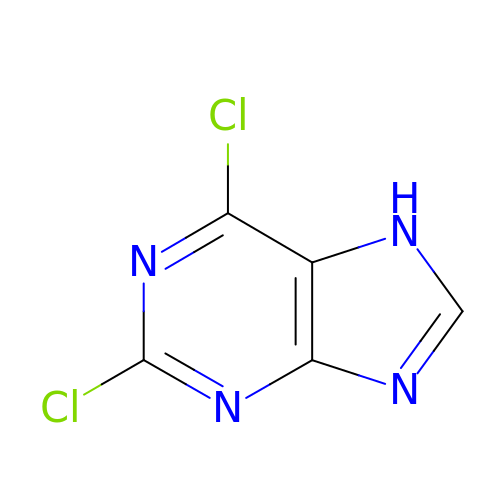2,6-bis(chloranyl)-7H-purine | C5 H2 Cl2 N4 | RMFWVOLULURGJI-UHFFFAOYSA-N>[4x]GSHMRAMNDRLPSFCTPLDDRWPLPVALPGVQLRSTRFDPALLQPGDFALAGIQPPANILRAVAKRQAEF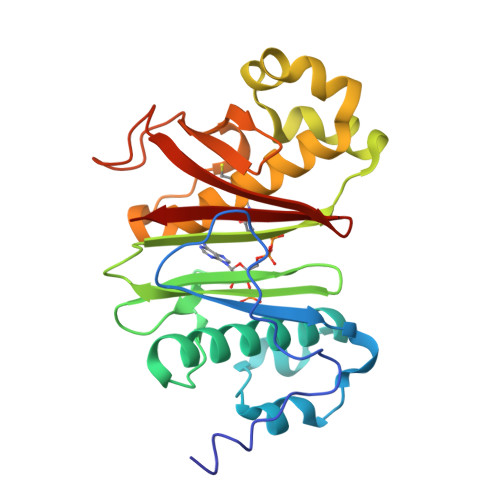LAGRLCARAALFALDGRAQTPAVGEDRAPVWPAAISGSITHGDRWAAALVAARGDWRGLGLDVETLLEAERARYLHGEILTEGERLRFADDLERRTGLLVTLAFSLKESLFKALYPLVGKRFYFEHAELLEWRADGQARLRLLTDLSPEWRHGSELDAQFAVLDGRLLSLVAVGA>[6x]MAAKVFESIGKFGLALAVAGGVVNSALYNVDAGHRAVIFDRFRGVQDIVVGEGTHFLIPWVQKPIIFDCRSRPRNVPVITGSKDLQNVNITLRILFRPVASQLPRIFTSIGEDYDERVLPSITTE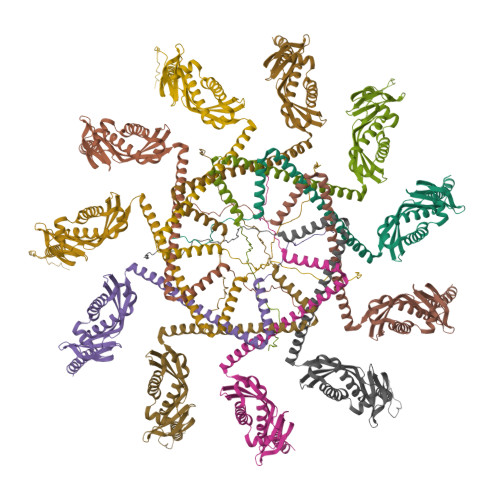ILKSVVARFDAGELITQRELVSRQVSDDLTERAATFGLILDDVSLTHLTFGKEFTEAVEAKQVAQQEAERARFVVEKAEQQKKAAIISAEGDSKAAELIANSLATAGDGLIELRKLEAAEDIAYQLSRSRNITYLPAGQSVLLQLPQ;>[5x]MAQNLKDLAGRLPAGPRGMGTALKLLLGAGAVAYGVRESVFTVEGGHRAIFFNRIGGVQQDTILAEGLHFRIPWFQYPIIYDIRARPRKISSPTGSKDLQMVNISLRVLSRPNAQELPSMYQRLGLDYEERVLPSIVNEVLKSVVAKFNASQLITQRAQVSLLIRRELTERAKDFSLILDDVAITELSFSREYTAAVEAKQVAQQEAQRAQFLVEKAKQEQRQKIVQAEGEAEAAKMLGEALSKNPGYIKLRKIRAAQNISKTIATSQNRIYLTADNLVLNLQDESFTRGSDSLIKGKK> SRLDII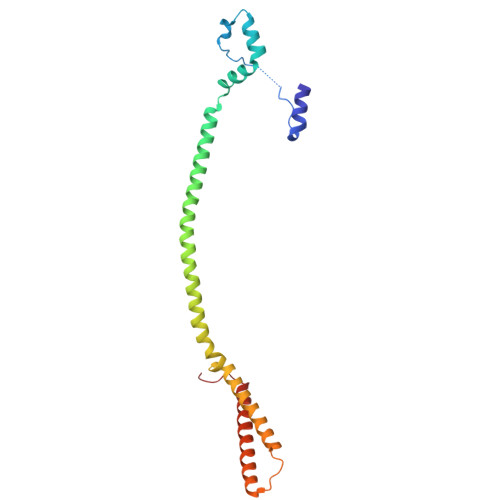RAEMDVVPSPGLPEKVNEKSKNIPLPEGINLLSSKEIIDLIQTHRHQLELYVTKFNPLTDFAGKIHAFRDQFKQLEENFEDLHEQKDKVQALLENARILESKYVASWQDYHSEFSKKYGDIALKKKLEQNTKKLDEESSQLETTTRSIDSADDLDQFIKNYLDIRTQYHLRREKLATWDKQGNLKY> TNLMVSTAVEKKKYLDSEFLLHCISAQLLDMWKQARARWLELVGKEWAHMLALNPERKDFLWKNQS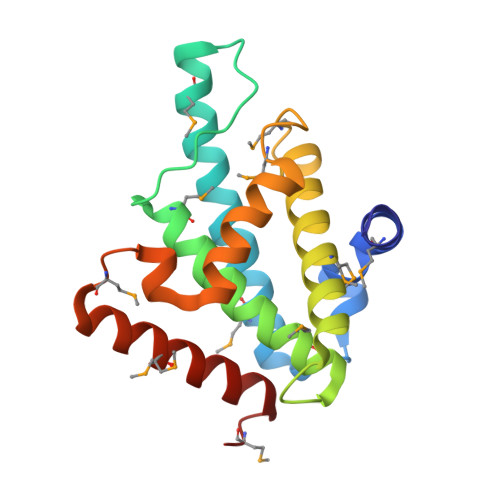EMNSAFFDLCEVGKQVMLGLLGKEVALPKEEQAFWIMYAVHLSAACAEELHMPEVAMSLRKLNVKLKDFNFGGTRYFKDMPPEEKKRRMERKQRIEEARRHGMP2',3'- 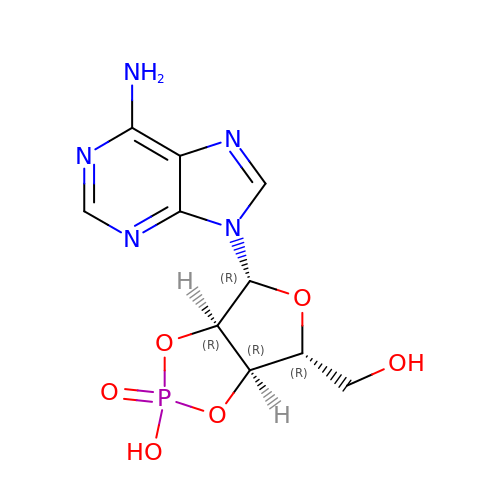cyclic AMP | C10 H12 N5 O6 P | KMYWVDDIPVNLME-KQYNXXCUSA-N> QPQFNEDTLQQRLQALIESAGENWTYAIFWQISHDFDSSTGDNTVILGWGDGYYKGEEDKEK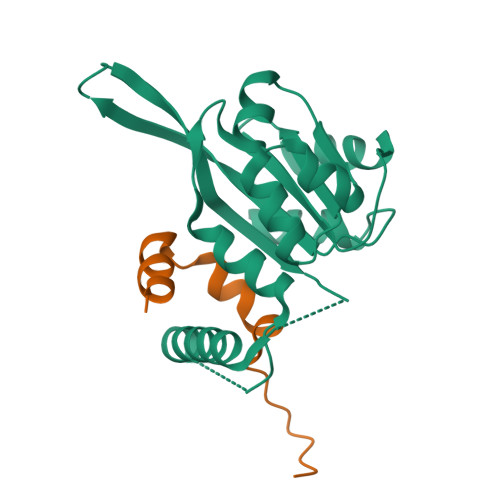KKNNTNTAEQEHRKRVIRELNSLISGGIGVSDESNDEEVTDTEWFFLVSMTQSFVNGVGLPGESFLNSRVIWLSGSGALTGSGCERAGQGQIYGLKTMVCIATQNGVVELGSSEVISQSSDLMHKVNNLFNFNNGGG;> KQTNNAPKPKFQKFLDRRRSFRDIQGAISKIDPEIIKSLLAST>[4x]MNEMLKHEYVKVNGIKMHYVTQGKGKLLLLLHGFPD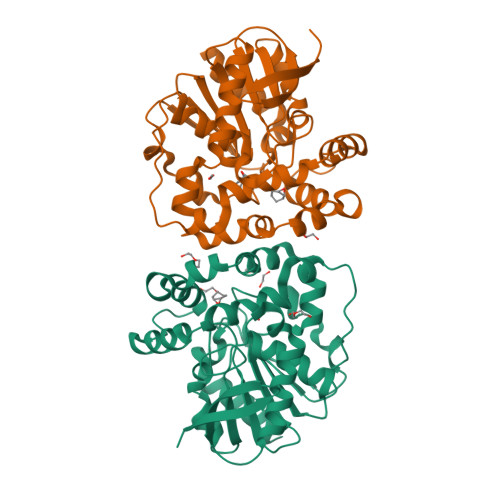FWYVWRFQIPALAKHFRVVAPDLRGYNETDKPEGVENYRLDLLAKDILGLIKALGEEHAVVVGHDWGGIISWTLTAFNPQAVEKLVILNAPHPKAYMTRTKNSLRQLQKSWYVFFFQVANIPEKILSRNEFAFLKNMLIQSFVRRDLLTEEDLRIYVDAWSKSGALTSALNYYRANLNPDIIFSEKTVVFPKIKVPTLVIWGEKDVAISKDLIVNMEDFIEAPYSIKYFPECGHWVQLEEPELVRKHIEEFILKSDIHHHHHH> REFTIDFSTQQSYVSSLNSIRTEISTPLEHISQGTTSVSVI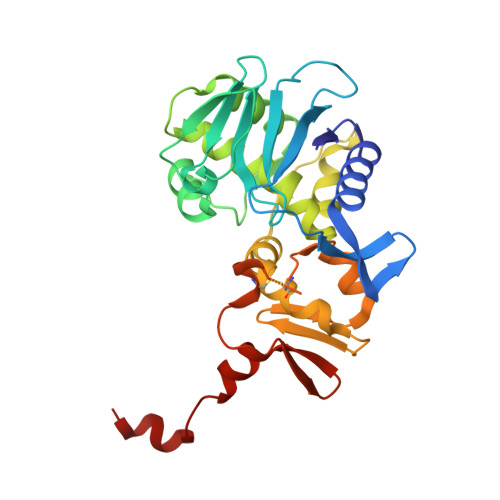NHTPPGSYFAVDIRGLDVYQARFDHLRLIIEQNNLYVAGFVNTATNTFYRFSDFTHISVPGVTTVSMTTDSSYTTLQRVAALERSGMQISRHSLVSSYLALMEFSGNTMTRDASRAVLRFVTVTAEALRFRQIQREFRQALSETAPVYTMTPGDVDLTLNWGRISNVLPEYRGEDGVRVGRISFNNISAILGTVAVILNCHHQGARSVRAVNEESQPECQITGDRPVIKINNTLWESNTAAAFLNRKSQFLYTTGK> MKEFYLTVEQIGDSIFERYIDSNGRERTREVEYKPSLFAHCPESQATKYFDIYGKPCTRKLFANMRDASQWIKRMEDIGLEALGMDDFKLAYLSDTYNYEIKYDHTKIRVANFDIEVT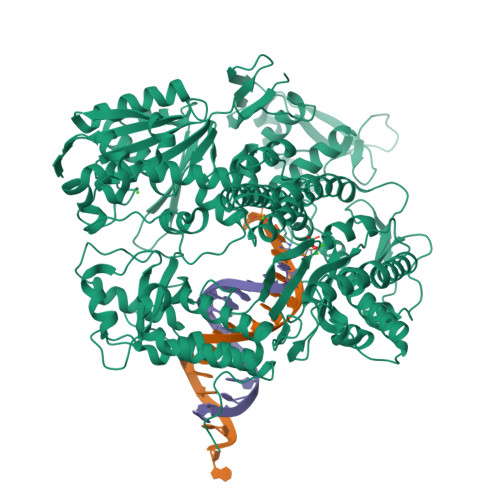SPDGFPEPSQAKHPIDAITHYDSIDDRFYVFDLLNSPYGNVEEWSIEIAAKLQEQGGDEVPSEIIDKIIYMPFDNEKELLMEYLNFWQQKTPVILTGWNVESFAIPYVYNRIKNIFGESTAKRLSPHRKTRVKVIENMYGSREIITLFGISVLDYIDLYKKFSFTNQPSYSLDYISEFELNVGKLKYDGPISKLRESNHQRYISYNIIAVYRVLQIDAKRQFINLSLDMGYYAKIQIQSVFSPIKTWDAIIFNSLKEQNKVIPQGRSHPVQPYPGAFVKEPIPNRYKYVMSFDLTSLYPSIIRQVNISPETIAGTFKVAPLHDYINAVAERPSDVYSCSPNGMMYYKDRDGVVPTEITKVFNQRKEHKGYMLAAQRNGEIIKEALHNPNLSVDEPLDVDYRFDFSDEIKEKIKKLSAKSLNEMLFRAQRTEVAGMTAQINRKLLINSLAGALGNVWFRYYDLRNATAITTFGQMALQWIERKVNEYLNEVCGTEGEAFVLYGDTDSIYVSADKIIDKVGESKFRDTNHWVDFLDKFARERMEPAIDRGFREMCEYMNNKQHLMFMDREAIAGPPLGSKGIGGFWTGKKRYALNVWDMEGTRYAEPKLKIMGLETQKSSTPKAVQKALKECIRRMLQEGEESLQEYFKEFEKEFRQLNYISIASVSSANNIAKYDVGGFPGPKCPFHIRGILTYNRAIKGNIDAPQVVEGEKVYVLPLREGNPFGDKCIAWPSGTEITDLIKDDVLHWMDYTVLLEKTFIKPLEGFTSAAKLDYEKKASL>SERFPNDVDPIETRDWLQAIESVIREEGVERAQYLIDQLLAEARKGGVNVAAGTGISNYINTIPVEEQPEYPGNLELERRIRSAIRWNAIMTVLRASKKDLELGGHMASFQSSATIYDVCFNHFFRARNEQDGGDLVYFQGHISPGVYARAFLEGRLTQEQLDNFRQEVHGNGLSSYPHPKLMPEFWQFPTVSMGLGPIGAIYQAKFLKYLEHRGLKDTSKQTVYAFLGDGEMDEPESKGAITIATREKLDNLVFVINCNLQRLDGPVTGNGKIINELEGIFEGAGWNVIKVMWGSRWDELLRKDTSGKLIQLMNETVDGDYQTFKSKDGAYVREHFFGKYPETAALVADWTDEQIWALNRGGHDPKKIYAAFKKAQETKGKATVILAHTIKGYGMGDAAEGKNIAHQVKKMNMDGVRHIRDRFNVPVSDADIEKLPYITFPEGSEEHTYLHAQRQKLHGYLPSRQPNFTEKLELPSLQDFGALLEEQSKEISTTIAFVRALNVMLKNKSIKDRLVPIIADEARTFGMEGLFRQIGIYSPNGQQYTPQDREQVAYYKEDEKGQILQEGINELGAGCSWLAAATSYSTNNLPMIPFYIYYSMFGFQRIGDLCWAAGDQQARGFLIGGTSGRTTLNGEGLQHEDGHSHIQSLTIPNCISYDPAYAYEVAVIMHDGLERMYGEKQENVYYYITTLNENYHMPAMPEGAEEGIRKGIYKLETIEGSKGKVQLLGSGSILRHVREAAEILAKDYGVGSDVYSVTSFTELARDGQDCERWNMLHPLETPRVPYIAQVMNDAPAVASTDYMKLFAEQVRTYVPADDYRVLGT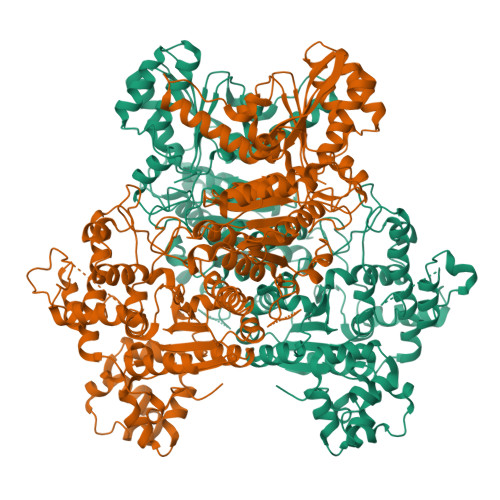DGFGRSDSRENLRHHFEVDASYVVVAALGELAKRGEIDKKVVADAIAKFNIDADKVNPRLA[2x]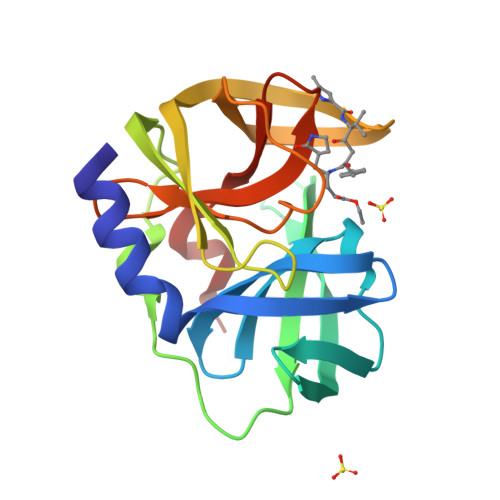> MGPSLDFALSLLRRNIRQVQTDQGHFTMLGVRDRLAVLPRHSQPGKTIWVEHKLVNVLDAVELVDEQGVDLELTLITLDTNEKFRDITKFIPENISTASDATLVINTEHMPSMFVPVGDVVQYGFLNLSGKPTHRTMMYNFPTKAGQCGGVVTSVGKVVGIHIGGNGRQGFCAGLKRSYFASEQ4-methoxyphenol | C7 H8 O2 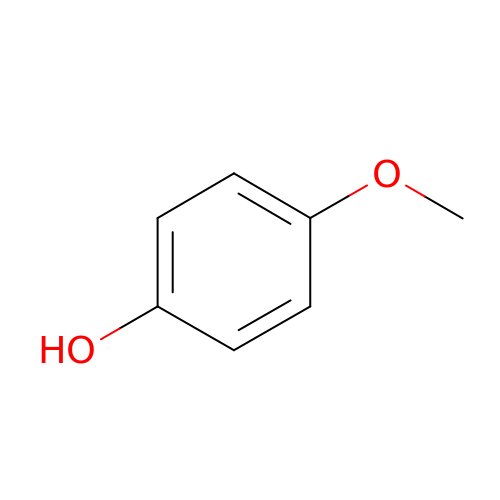| NWVVVBRKAWDGAB-UHFFFAOYSA-N STEP is a brain-specific PTP, and a validated therapeutic target for Alzheimer’s disease, Fragile X syndrome, and Parkinson’s disease. To compare the effects of temperature vs. pressure on the STEP catalytic domain, we used similarly prepared crystals to obtain three complementary crystal structures: one at cryogenic temperature (100 K) and ambient pressure (0.1 MPa), one at physiological temperature (310 K) but ambient pressure, and one at high pressure (205 MPa) but cryogenic temperature via high-pressure cryocooling. For the remainder of this paper, we refer to the structure at low temperature and low pressure as LoTP, the structure at high temperature as HiT, and the structure at high pressure as HiP. All three structures have the expected PTP catalytic domain architecture, including several key loops surrounding the active site region.

One notable feature of our new structures differs from the previous STEP structures: the active site binds two sulfate molecules. The bottom sulfate is well-coordinated by the catalytic P loop, analogous to the phosphate group in the phosphotyrosine (pTyr) substrate in PDB ID 2cjz41. In our structures, as supported by strong electron density, Cys472 predominantly adopts a side-chain rotamer that points away from the sulfate, thus avoiding a steric clash. Taken together, these observations support the interpretation that Cys472 samples both a rare primary rotamer and a low-occupancy alternate rotamer that is sterically mutually exclusive with a fortuitously observed sulfate bound at high but non-unity occupancy. Thus, although previous structures of STEP have sulfates or phosphate-like chemical groups independently in each of these sites, no previous structure has them in both sites simultaneously. In our manually modeled, deposited structures, LoTP has by far the most waters, HiT has by far the fewest, and HiP has an intermediate number. First, at LoTP and HiP, an ordered glycerol molecule is bound near α2′ and the Q loop. By contrast, at HiT, ordered waters are present instead, and α1′-α2′ and the Q loop undergo conformational shifts. Importantly, all three structures are from crystals treated with similar glycerol-containing cryoprotectant solutions. It is thus plausible that crystal cryocooling induces the glycerol to bind, preventing nearby conformations with potential functional relevance seen at physiological temperature.

> SMSRVLQAEELHEKALDPFLLQAEFFEIPMNFVDPKEYDIPGLVRKNRYKTILPNPHSRVCLTSPDPDDPLSSYINANYIRGYGGEEKVYIATQGPIVSTVADFWRMVWQEHTPIIVMITNIEEMNEKCTEYWPEEQVAYDGVEITVQKVIHTEDYRLRLISLKSGTEERGLKHYWFTSWPDQKTPDRAPPLLHLVREVEEAAQQEGPHCAPIIVHCSAGIGRTGCFIATSICCQQLRQEGVVDILKTTCQLRQDRGGMIQTCEQYQFVHHVMSLYEKQLSH> MDYKDHDGDYKDHDIDYKDDDDKGGRMEGSTGFDGDATTFFAPDAVFGDRVRRFQEFLDTFTSYRDSVRSIQVYNSNNAANYNDDQDDADERDLLGDDDGDDLEKEKKAASSTSLNILPHRIIISLDDLREFDRSFWSGILVEPAYFIPPAEKALTDLADSMDDVPHPNASAVSSRHPWKLSFKGSFGAHALSPRTLTAQHLNKLVSVEGIVTKTSLVRPKLIRSVHYAAKTGRFHYRDYTDATTTLTTRIPTPAIYPTEDTEGNKLTTEYGYSTFIDHQRITVQEMPEMAPAGQLPRSIDVILDDDLVDKTKPGDRVNVVGVFKSLGAGGMNQSNSNTLIGFKTLILGNTVYPLHARSTGVAARQMLTDFDIRNINKLSKKKDIFDILSQSLAPSIYGHDHIKKAILLMLMGGVEKNLENGSHLRGDINILMVGDPSTAKSQLLRFVLNTASLAIATTGRGSSGVGLTAAVTTDRETGERRLEAGAMVLADRGVVCIDEFDKMTDVDRVAIHEVMEQQTVTIAKAGIHTTLNARCSVIAAANPVFGQYDVNRDPHQNIALPDSLLSRFDLLFVVTDDINEIRDRSISEHVLRTHRYLPPGYLEGEPVRERLNLSLAVGEDADINPEEHSNSGAGVENEGEDDEDHVFEKFNPLLQAGAKLAKNKGNYNGTEIPKLVTIPFLRKYVQYAKERVIPQLTQEAINVIVKNYTDLRNDDNTKKSPITARTLETLIRLATAHAKVRLSKTVNKVDAKVAANLLRFALLGEDIGNDIDEEE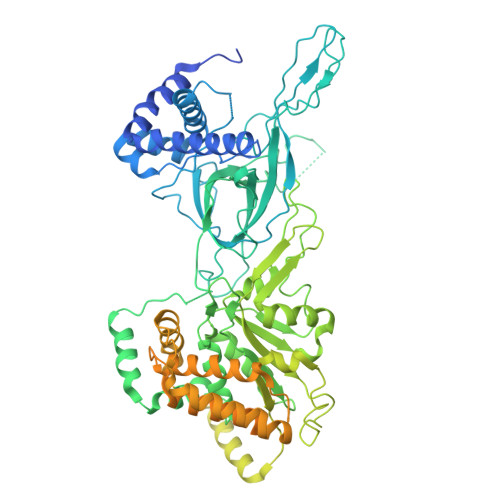SEYEEALSKRSPQKSPKKRQRVRQPASNSGSPIKSTPRRSTASSVNATPSSARRILRFQDDEQNAGEDDNDIMSPLPADEEAELQRRLQLGLRVSPRRREHLHAPEEGSSGPLTEVGTPRLPNVSSAGQDDEQQQSVISFDNVEPGTISTGRLSLISGIIARLMQTEIFEEESYPVASLFERINEELPEEEKFSAQEYLAGLKIMSDRNNLMVADDKVWRV> GAMGSGASSQ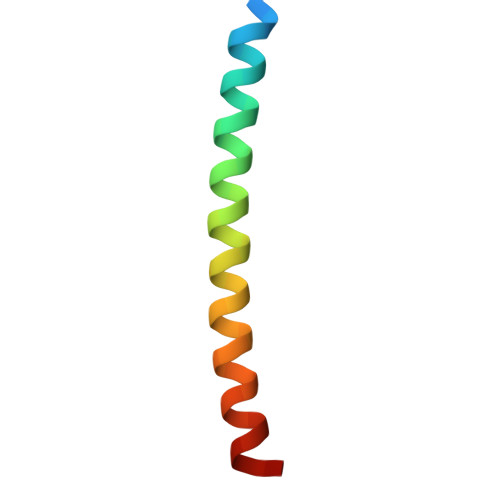AACLKQILLLQLDLIEQQQQQLQAKEKEIEELKS> MTGREILEKLERREFTREVLKEALSINDRGFNEALFKLADEIRRKYVGDEVHIRAIIEFSNVCRKNCLYCGLRRDNKNLKRYRMTPEEIVERARLAVQFGAKTIVLQSGEDPYXMPDVISDIVKEIKKMGVAVTLSLGEWPREYYEKWKEAGADRYLLRHETANPVLHRKL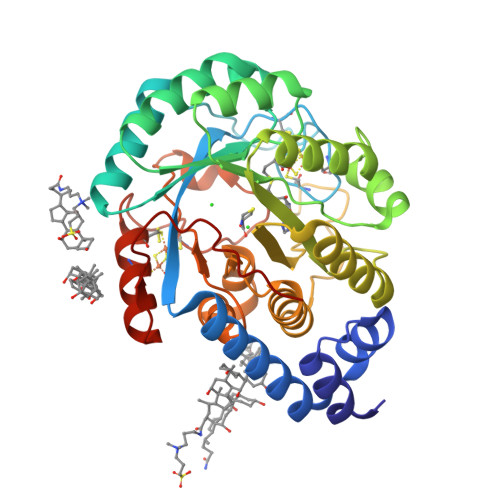RPDTSFENRLNCLLTLKELGYETGAGSMVGLPGQTIDDLVDDLLFLKEHDFDMVGIGPFIPHPDTPLANEKKGDFTLTLKMVALTRILLPDSNIPATTAMGTIVPGGREITLRCGANVIMPNWTPSPYRQLYQLYPGKICVFEKDTACIPCVMKMIELLGRKPGRDWGGRKRVFETV>MGHHHHHHHMDNAIGKPSLPRASRLDGQATRLQILEKAGELFAEQGLANTTSKQICERSQANSAAVNYHFVNKEGLYRAVLLEAHARLVQLETLVSLNERPGSPQDKLRALITVLVERLHNHPDGWALKVLTREVLSPSPEFEVVLKEQSFPKAHILRGLLGQIMNLPADHPT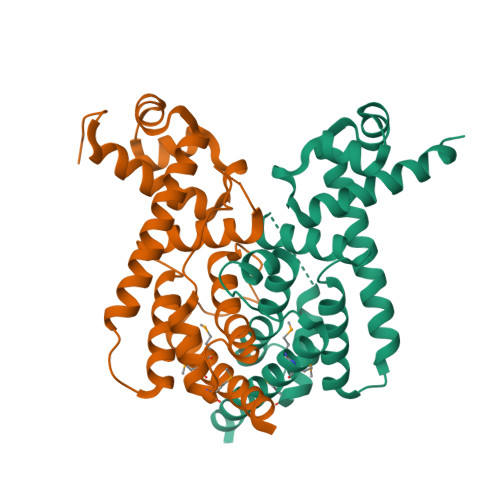TLRSAISVFAPCLFLLIAHQPLKQHVLQGLSLEPQGLIDHMMSYALGGLQAVAATAHDAAS[2x]>MNIQAIDTRHGTANQHSFSNGNCLPYTGVPFGMNFYAPQTT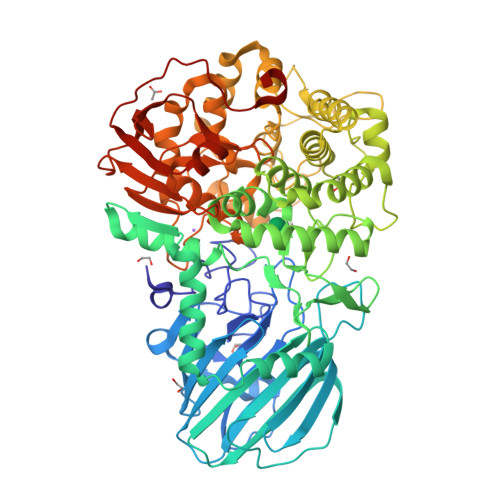DQKGSWWFHPEDRTFQGYRVTHQPSPWMGDFSHLLMTPVSGSLSELSLFHAQSSYRPEESLFSPVEINLTQLRYQITSQLIPSMYGGILTIDYQQKDNHLLLTLPGRYQVKQLDDHQVAVKVINYSGCEDPDFSFYFVLHFEQPLTKWFAPSSGEDGKILLSFGNIAQQVVHFSSSFISEKQAQLNLAREISLRSTEMLQQGIADWHNYFDRLKVTHENPEHTKTFYHTLYRTFLFPQTFYELDENQQPIHYDTFSQTVRPGVLYTNNGFWDTYKTVYPLFSLIAQEKYEEMLEGFLNSYNETGFLPKWLSPDERGLMPGTLIDAVIADAAVKKIRPDLMPQFLEAMKKGATQQSERENYGRQGTLDYLKYGYVPSTYHESVNHTLDYAYSDFCISQVAKTLNDSETATFYRQQALNYQQLFNPETGFMQAKDTEGNFRPDFLDIRWGKDYAEGSAWQSSFAVYQDFAGLIKLYGSELAFEKKLIQLCNQAPNFNVEGYGFEIHEMSEMAAIDFGQLAISNQPSFHYPFLFSYIGKPEMAQPLLKQLMQTFDASPTGYPGDEDNGSMSAWYIFNSLGFYPVTPGAGEYVIGMPLVQTAEVKLSNGKQLTIQTSPNKVQQQFIHEIQLNQEKHTAPYFTHQELLNGGTLDYQLGIVPNPQTTAERPFSLSTEKLEHHHHHH[4x]> SRCTHLENRDFVTGTQGTTRVTLVLELGGCVTITAEGKPSMDVWLDAIYQENPAQTREYCLHAKLSDTKVAARCPTMGPATLAEEHQGGTVCKRDQSDRGWGNHCGLFGKGSIVACVKAACEAKKKATGHVYDANKIVYTVKVEPHTGDYVAANETHSGRKTASFTVSSEKTILTMGEYGDVSLLCRVASGVDLAQTVILELDKTVEH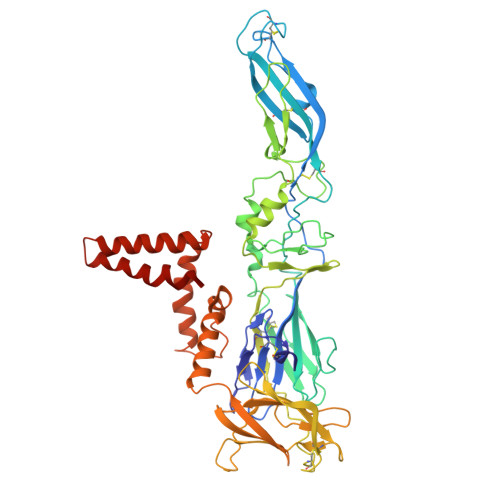LPTAWQVHRDWFNDLALPWKHEGARNWNNAERLVEFGAPHAVKMDVYNLGDQTGVLLKALAGVPVAHIEGTKYHLKSGHVTCEVGLEKLKMKGLTYTMCDKTKFTWKRAPTDSGHDTVVMEVTFSGTKPCRIPVRAVAHGSPDVNVAMLITPNPTIENNGGGFIEMQLPPGDNIIYVGELSYQWFQKGSSIGRVFQKTKKGIERLTVIGEHAWDFGSAGGFLSSIGKALHTVLGGAFNSIFGGVGFLPKLLLGVALAWLGLNMRNPTMSMSFLLAGVLVLAMTLGVGA> GIGTGFPFDPHYVEVLGERMHYVDVGPRDGTPVLFLHGNPTSSYVWRNIIPHVAPTHRCIAPDLIGMGKSDKPDLGYFF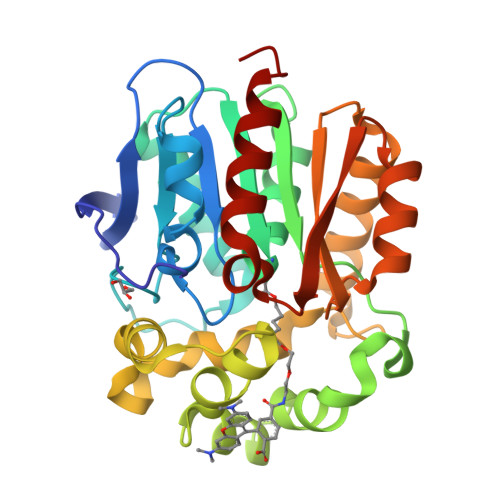DDHVRFMDAFIEALGLEEVVLVIHDWGSALGFHWAKRNPERVKGIAFMEFIRPIPTWDEWPEFARETFQAFRTTDVGRKLIIDQNVFIEGTLPMGVVRPLTEVEMDHYREPFLNPVDREPLWRFPNELPIAGEPANIVALVEEYMDWLHQSPVPKLLFWGTPGVLIPPAEAARLAKSLPNCKAVDIGPGLNLLQEDNPDLIGSEIARWLSTLEI>[8x]M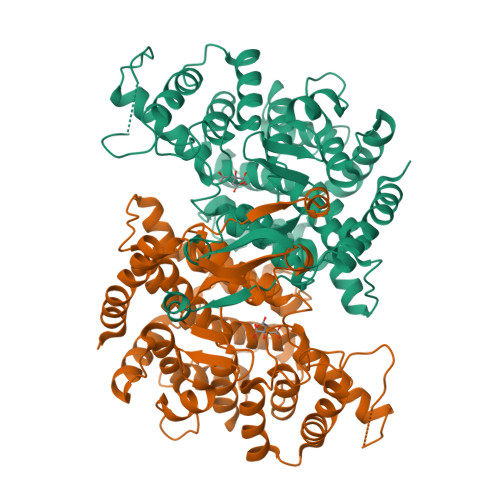SFLKEKLAEKIAQHRPRTTRLLKEFGNVKIDEVTISQAIGGMRGIKSLVTDISYLDPEEGIRFRGYTIPEVLEKLPKVPGAEMPYVEGHFYLLLTGDVPTEKEVKEVAEEFKKRRALPEYVKDTLKAMPRDTHPMTMFAAGILAMQRESKFAAYYNAGKFNKNTAWEPMFEDAMDLMAKLPSLGAYIYRMKYKSDTHIPSNPDLDLGGDFANMMGIDKPYDDVARLYFILHSDHESGNVSAHTAHLVASALSDAYYAYSAAMCGLAGPLHGLANQEVLKWIQETIDKKLGGKVPTKEELKKFVEETLSSGQVIPGYGHAVLRKTDPRYVAQREFALKHMPDDPIFQVVSMLYEVVPPILSSLGKVKDPWPNVDAHSGCIQWHYGVVEYDFYTVLFGIGRALGVLANLVWDRALGYAIERPKSVTTDMLEKWAGIK>[4x]SAKAAEGYEQIEVDVVAVWKEGYVYENRGSTSVDQKITITKGMKNVNSETRTVTATHSIGSTISTGDAFEIGSVEVSYSHSHEESQVSMTETEVYESKVIEHTITIPPTSKFTRWQLNADVGGADIEYMYLIDEVTPIGGTQSIPQVITSRAKIIVGRQIILGKTEIRIKHAERKEYMTVVSRKSWPAATLGHSK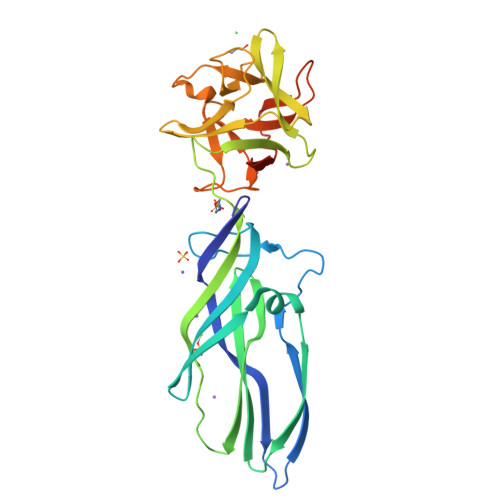LFKFVLYEDWGGFRIKTLNTMYSGYEYAYSSDQGGIYFDQGTDNPKQRWAINKSLPLRHGDVVTFMNKYFTRSGLCYDDGPATNVYCLDKREDKWILEVVGLVPRGSGHHHHHH> GSNNVLPTWSLDSNGEMRSRLSLSEVLDSGDLMKFAVDKTGCQFLEKAVKGSLTSYQKFQLFEQVIGRKDDFLKLSTNIFGNYLVQSVIGISLATNDDGYTKRQEKLKNFISSQMTDMCLDKFACYVIQSSLQNMDLSLACKLVQALPRDARLIAICVDQNANHVIQKVVAVIPLKNWEFIVDFV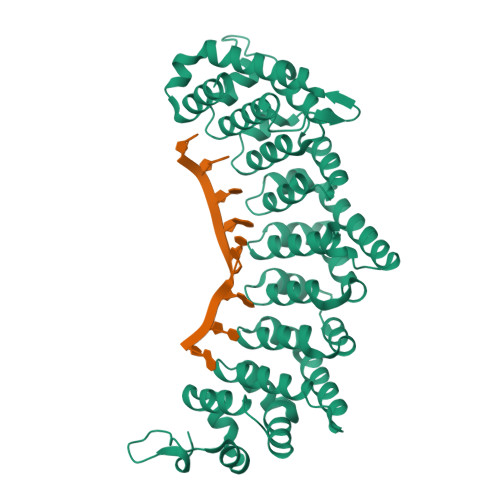ATPEHLRQICSDKYGCRVVQTIIEKLTADSMNVDLTSAAQNLRERALQRLMTSVTNRCQELATNEYANYIIQHIVSNDDLAVYRECIIEKCLMRNLLSLSQEKFASHVVEKAFLHAPLELLAEMMDEIFDGYIPHPDTGKDALDIMMFHQFGNYVVQCMLTICCDAVSGRRQTKEGGYDHAISFQDWLKKLHSRVTKERHRLSRFSSGKKMIETLANLRSTHPIYELQ> MDEFEMIKRNTSEIISEEELREVLKKDEKSAGIGF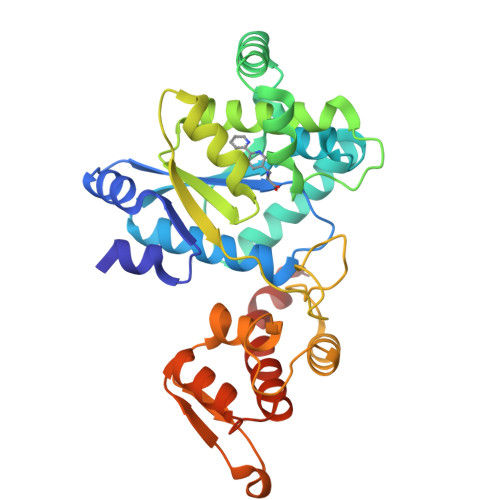EPSGKIHLGHYLQIKKMIDLQNAGFDIIIYLADLAAYLNQKGELDEIRKIGDYNKKVFEAMGLKAKYVYGSEFQLDKDYTLNVYRLALKTTLKRARRSMELIAREDENPKVAEVIYPIMEVNGWHYSGVDVAVGGMEQRKIHMLARELLPKKVVCIHNPVLTGLDGEGKMSSSKGNFIAVDDSPEEIRAKIKKAYCPAGVVEGNPIMEIAKYFLEYPLTIKRPEKFGGDLTVNSYEELESLFKNKELHPMDLKNAVAEELIKILEPIRKRLLEHHHHHH> MWPPRLLSCIFTIILIVAVIAPTSDSTTVRRRLRKPSKSVSVTSSVSRSTDQVISASVNRPKIRGRPSVASRKSSAALDNSVGTDDHKDKDGYKIVCYYTNWSQYRTKIGKFMPEDIQPELCTHIIFAFGWLKKGKLSSFESNDETKDGKTGLYDRINALKKANPKLKTLLAIGGWSFGTQKFKEMSATRYARQTFIYSAIPYLRDRNFDGLDIDWEYPKGGDDKKNYVLLLKELREAFEAEAQEVKKPRLLLTAAVPVGPDNIKSGYDVPAVASYLDFINLMAYDFHGKWERETGHNAPLYAPSSDSEWRKQLSVDHAAHLWVKLGAPKEKLIIGMPTYGRTFTLSNPNNFKVNSPASGGGKAGEYTKESGFLAYYEVCEILRNGGAYVWDDEMKVPYAIHGDQWVGFDDEKSIRNKMRWIKDNSFGGAMVWTVDMDDFSGGVCGGNVKYPLIGAMREELRGISRGKDAKDVDWASVAASV

Here, we report an arthropod-conserved insect chitinase belonging to group III from the pest Ostrinia furnacalis (OfChtIII), which contains two GH18 domains that act without synergism according to enzymatic assays and structural investigations. OfChtIII contains 987 amino-acid residues and is composed of four domains: a predicted TM domain (residues 7–29), two catalytic domains, GH18A (residues 94–461) and GH18B (residues 530–889), and a CBM14 domain (residues 922–976). The two GH18 domains of OfChtIII possess similar structures and substrate specificities, which differentiate them from the chitinolytic chitinase OfChtI-CAD. The degradation activity of GH18A and GH18B (or GH18B-CBM14) in combination towards EGC was equal to the activity calculated from the sum of the individual activities, suggesting that there was no synergistic effect between them.

GH18A crystallized in space group P41212, and the structure was determined by molecular replacement using human AMCase as a template. The structures of the complexes were determined by molecular replacement using GH18A as a template. These structures were resolved to resolutions of between 2.0 and 3.0 Å and all data-collection and structure-refinement statistics are summarized in Table 2. A unique loop (residues 145–152) is adjacent to the α7 helix. Additionally, a substrate-binding groove with lined-up aromatic residues is located on the surface. Secondly, the structures of GH18A and GH18B are very similar, with an r.m.s.d. of 0.88 Å for 344 Cα atoms. Although the overall structures of GH18A and GH18B are similar to that of OfChtI-CAD, with r.m.s.d.s of 1.3 Å (for 367 Cα atoms) and 1.5 Å (for 360 Cα atoms), respectively, there are obvious differences between the two enzymes. Firstly, GH18A and GH18B from OfChtIII do not have the same surface hydrophobic planes as found in the GH18 domain of OfChtI (characterized by Phe159, Phe194, Trp241 and Tyr290). Secondly, both GH18 domains have shorter and shallower substrate-binding clefts than OfChtI-CAD. As calculated by the CASTp software with default parameters, the volumes of the substrate-binding clefts of OfChtI-CAD, GH18A and GH18B were estimated to be 1628, 1399 and 1100 Å3, respectively.> MSLYLFMLFLQPLSLSFVS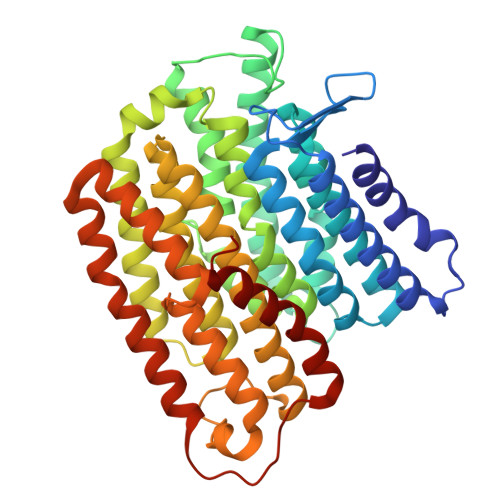RSFSKISSLMMSFATLWSAVYMWFTSNGANQTFYQVVSWGSDWSTFGVCYTSLYISLLCAFIFPICVILVQGYRALSILICIQTAVSLSIVSLHMLAFYALFESSLLLFFILIGRRKYGSLSAAYNISIYTFISALGFLISAFWLNWSFGSVCALLPNEEANSFVAFGIFILLWVKAPLVPFHLWLPEAHVYAPTAGSVLLAGVLLKISIVGLHVFFLPICASSIVKAFPLILSICLGSFIFSSFSTLKQIDLKKIVAYSSISHMAIVFLSSATNSGLGIQGAVLYCIAHGLISPGLFLLVGILYKNTNTKLVFYLRGLSQQAPVWWSVWVFFMLGNLAFPLFPNFIAEVVCLSALFKNHELYAYAFIFFSFVGTVYSSTVLGRLKGGVSSQCVDASRLDVISWNPLVLATVVTGIGYM> MAYNENDFKYFDDIRPFLDEIYKTRERYTPFYDDRADYNTNSKSYYDYISRLSKLIEVLARRIWDYDNELKKRFKNWDDLMKAFPEQAKDLFRGWLNDGTIDSIIHDEFKKYSAGLTSAFALFKVTEMKQMNDFKSEVKDLIKDIDRFVNGFELNELEPKFVMGFGGIRNAVNQSINIDKETNHMYSTQSDSQKPEGFWINKLTPSGDLISSMRIVQGGHGTTIGLERQSNGEMKIWLHHDGVAKLLQVAYKDNYVLDLEEAKGLTDYTPQSLLNKHTFTPLIDEANDKLILRFGDGTIQVRSRADVKNHIDNVEKEMTIDNSENNDNRWMQGIAVDGDDLYWLSGNSSVNSHVQIGKYSLTTGQKIYDYPFKLSYQDGINFPRDNFKEPEGICIYTNPKTKRKSLLLAMTNGGGGKRFHNLYGFFQLGEYEHFEALRARGSQNYKLTKDDGRALSIPDHIDDLNDLTQAGFYYIDGGTAEKLKNMPMNGSKRIIDAGCFINVYPT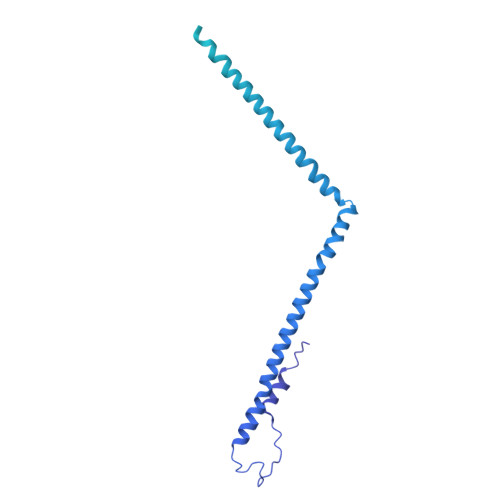TQTLGTVQELTRFSTGRKMVKMVRGMTLDVFTLKWDYGLWTTIKTDAPYQEYLEASQYNNWIAYVTTAGEYYITGNQMELFRDAPEEIKKVGAWLRVSSGNAVGEVRQTLEANISEYKEFFSNVNAETKHREYGWVAKHQK> MINGVYYNEISRDLDISSSTQCLRFLKETVIPSLANNGNNSTSIQYHGISKNDNIKKSVNKLDKQINMADRSLGLQQVVCIFSYGPHIQKMLSILEIFKKGYIKNNKKIYQWNKLTSFDIKREGRNELQEERLKVPILVTMVSDSEIIDLNLHSFTKQ;> MALKKNTHNKSTKRVTKHPSLKTLTHKQ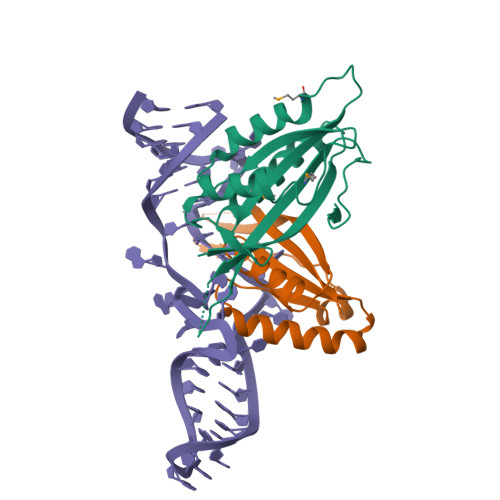IHTTIFVKSTTPYVSALKRINKFLDSVHKQGSSYVAVLGMGKAVEKTLALGCHFQDQKNKKIEVYTKTIEVLDEVITEGQADIDMESDVEDDDKETQLKKRAVSGVELRIYV> TLLSPKGSISEETKQKLKSAILSAQSA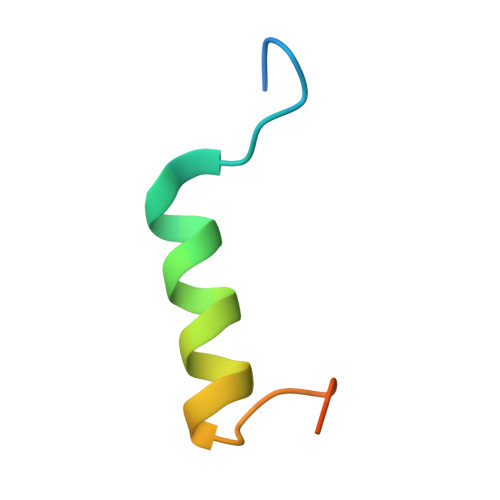ANVRKESL>MHHHHHHDSKHQCVKLNDGHFMPVLGFGTYAPPEVPRSKALEVTKLAIEAGFRHIDSAHLYNNEEQVGLAIRSKIADGSVKREDIFYTSKLWSTFHRPELVRPALENSLKKAQLDYVDLYLIHSPMSLKPGEELSPTDENGKVIFDIVDLCTTWEAMEKCKDAGLAKSIGVSNFNRRQLEMILNKPGLKYKPVCNQVECHPYFNRSKLLDFCKSKDIVLVAYSA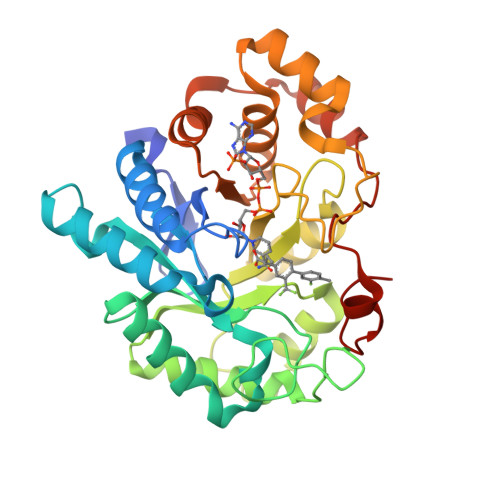LGSQRDKRWVDPNSPVLLEDPVLCALAKKHKRTPALIALRYQLQRGVVVLAKSYNEQRIRQNVQVFEFQLTAEDMKAIDGLDRNLHYFNSDSFASHPNYPYSDEY[2x]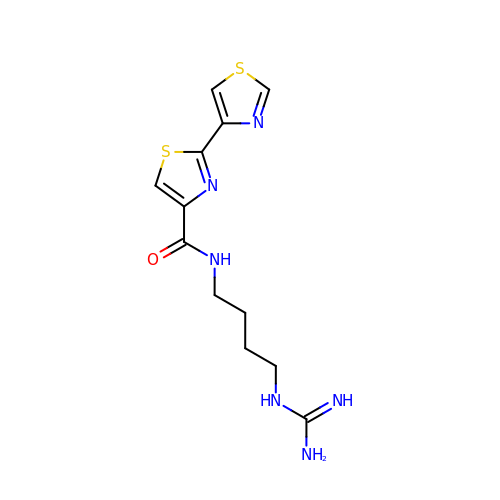N-(4-{[amino(imino)methyl]amino}butyl)-2,4'-bi-1,3-thiazole-4-carboxamide | C12 H16 N6 O S2 | VSIFMASDYAMOAN-UHFFFAOYSA-N>[2x]MVLYFIGLGLYDERDITVKGLEIAKKCDYVFAEFYTSLMAGTTLGRIQKLIGKHIRVLSREDVELNFENIVLPLAKENDVAFLTPGDPLVATTHAELRIRAKRAGVESYVIHAPSIYSAVGITGLHIYKFGKSATVAYPEGNWFPTSYYDVIKENAERGLHTLLFLDIKAEKRMYMTANEAMELLLKVEDMKKGGVFTDDTLVVVLARAGSLNPTIRAGYVK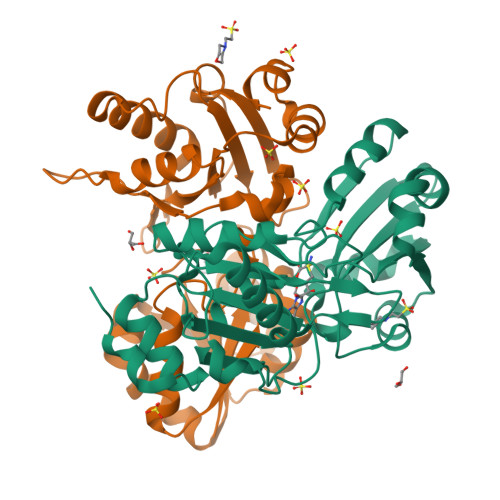DLIREDFGDPPHILIVPGKLHIVEAEYLVEIAGAPREILRVNV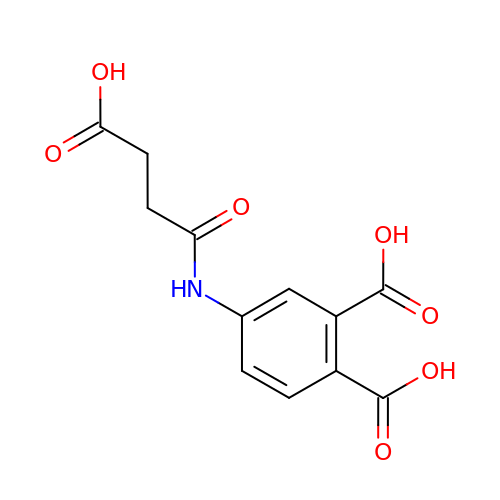4-[(3-carboxypropanoyl)amino]benzene-1,2-dicarboxylic acid | C12 H11 N O7 | JVZSGTXFIVTSIN-UHFFFAOYSA-N> MWDVIDLSRWQFALTALYHFLFVPLTLGLIFLLAIMETIYVVTGKTIYRDMTRFWGKLFGINFALGVATGLTMEFQFGTNWSFYSNYVGDIFGAPLAMEALMAFFLESTFVGLFFFGWQRLNKYQHLLVTWLVAFGSNLSALWILNANGWMQYPTGAHFDIDTLRMEMTSFSELVFNPVSQVKFVHTVMAGYVTGAMFIMAISAWYLLRGRERNVALRSFAIGSVFGTLAIIG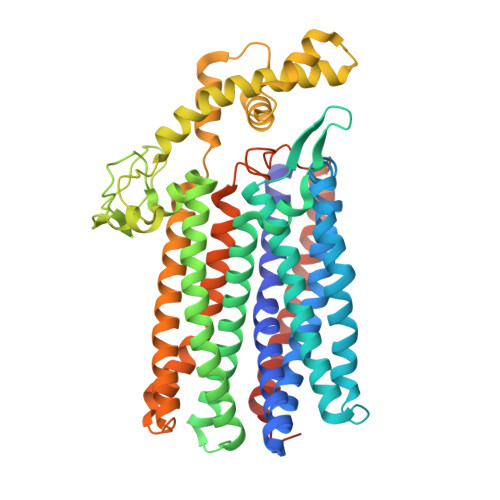TLQLGDSSAYEVAQVQPVKLAAMEGEWQTEPAPAPFHVVAWPEQDQERNAFALKIPALLGILATHSLDKPVPGLKNLMAETYPRLQRGRMAWLLMQEISQGNREPHVLQAFRGLEGDLGYGMLLSRYAPDMNHVTAAQYQAAMRGAIPQVAPVFWSFRIMVGCGSLLLLVMLIALVQTLRGKIDQHRWVLKMALWSLPLPWIAIEAGWFMTEFGRQPWAIQDILPTYSAHSALTTGQLAFSLIMIVGLYTLFLIAEVYLMQKYARLGPSAMQSEQPTQQQG>[8x]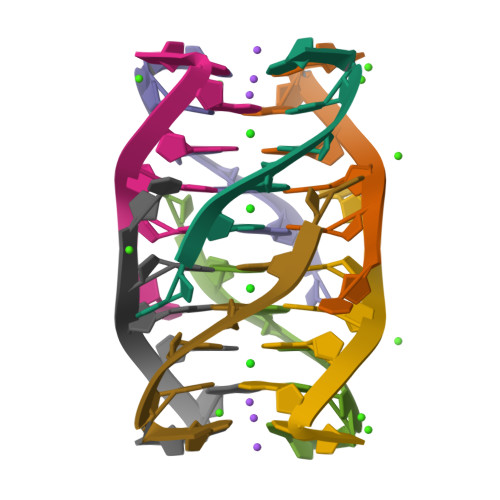UGGGGU> PCLYITTNVNFDGVNTDPFYSEVTKAVASIVGRPQNLVMVVLKGSVEIVFGGNKEAAAYAEIVSMGGITKQVKRELIATV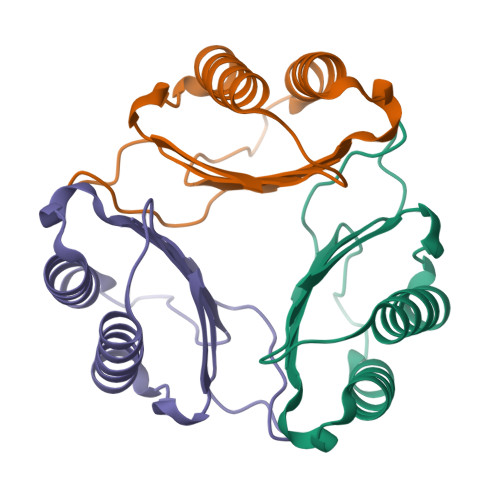GSILHTHFSIHPTRFIFKVF>GAMGSKPDTHRADERRFLDERGSSGPLAPNGLNPATIMEKAVRERIVESYFWKEQCFGVNEADIVDRVVEHVRFVGGVTGVTQKPSPFLCLAFKLLQLAPGDDILKEYLYFGGEKFKYLRALAAFYIRLTRPDKEVYTLLEPFLEDRRKLRRKGKNGTSLTYMDEFIDDLLTKDRVCSTSLWKMRRRDILEDLDLLEPRVSPLGSLEDILEEEEQAAKNEDGE[2x];>GAMGTTDDVDPEAEYAAWKLRELRRLRRERDAIEARERELAELERRRNLTEEERRA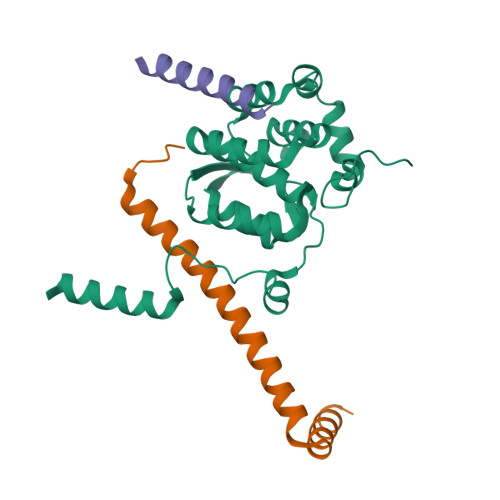EDEAHLAKQKAEKESRGKMGYLQKYFHR[2x];>GAGEVKKATAEEVHARIEFLWQREQEKKKEQVVSLK[2x]In alginate producing strains isolated from CF patients, the transcription factor AmrZ (Alginate and Motility Regulator Z, formerly AlgZ) is highly expressed. The 108 amino acid, 12.3 kD AmrZ protein is a member of the ribbon-helix-helix (RHH) family of DNA binding proteins, sharing highest sequence similarity to the Arc and Mnt repressors from bacteriophage P22. AmrZ and Helicobacter pylori NikR are currently the only characterized RHH proteins known to function as both transcriptional activators and repressors. AmrZ is necessary for alginate production, via the activation of algD, which is the first gene in the alginate biosynthetic operon.

We determined the structure of a C-terminal truncation mutant of AmrZ, Δ42, in complex with an 18 bp oligonucleotide containing the amrZ1 site to 3.1 Å resolution. The Δ42 variant of AmrZ (residues 1–66) contains the extended N-terminus and the RHH DNA binding domain, but has a truncated C-terminal domain. The structure reveals AmrZ binds the amrZ1 site as a dimer-of-dimers, and DNA recognition occurs by the interaction with two half sites on the DNA, separated by five base pairs. The dimer-dimer interface, which occludes approximately 290 Å2 of surface area on each dimer, is formed by a series of interactions between specific residues located on the loop connecting α-helix 1 and α-helix 2 on chains B and C. The insertion of the anti-parallel β-sheet from each AmrZ dimer into the major groove of the amrZ1 site provides for the recognition of two half sites, each with the sequence 5′-GGC (orange bases). Sequence dependent binding by AmrZ occurs via the interaction of three residues, Lys18, Val20, and Arg22, with the nucleotides. Lys18 from one AmrZ monomer is positioned where it can form hydrogen bonding interactions to the O6 and N7 atoms of the two guanine nucleotides, G23 and G24 (G4 and G5 on the other half site). The DNA binding β-sheet also orients the residue Arg22, from the other monomer of the dimer, to form a bidentate hydrogen bond to both the O6 and N7 atoms of the nucleotide G12 (G31 on the other half site). In the AmrZ structure, it appears that residue Val20 is poised to select for cytosine bases C13 and C14 (C32 and C33 on other half site) via a hydrophobic interaction. Residues 10–17 of the N-terminus form a looped structure, allowing the amino acids Ser13 and Arg14 in the major groove to interact with the DNA.

>[4x]GPHMRPLKQATPTYSSRTADKFVVRLPEGMREQIAEVARSHHRSMNSEIIARLEQSLLQEGALQDNLGV>MRGSHHHHHTTGEDDESECVINYVEKAVNKLTLQMPYQLFIGGEFVDAEGSKTYNTINPTDGSVICQVSLAQVSDVDKAVAAAKEAFENGLWGKINARDRGRLL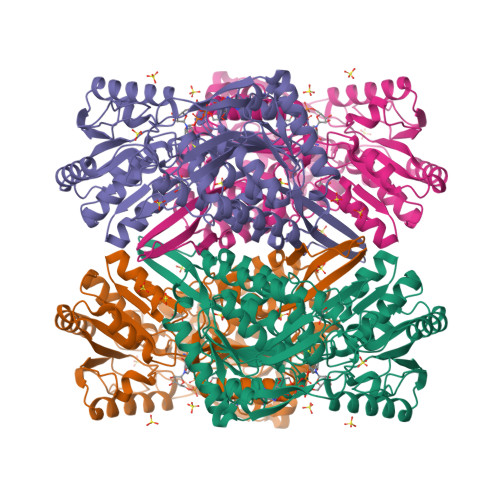YRLADVMEQHQEELATIEALDAGAVYTLALKTHVGMSIQTFRYFAGWCDKIQGATIPINQARPNRNLTLTKKEPVGVCGIVIPWNYPLMMLSWKTAACLAAGNTVVIKPAQVTPLTALKFAELTLKAGIPKGVVNILPGSGSLVGQRLSDHPDVRKIGFTGSTEVGKHIMKSCALSNVKKVSLELGGKSPLIIFADCDLNKAVQMGMSSVFFNKGENCIAAGRLFVEESIHNQFVQKVVEEVEKMKIGNPLERDTNHGPQNHEAHLRKLVEYCQRGVKEGATLVCGGNQVPRPGFFFQPTVFTDVEDHMYIAKEESFGPIMIISRFADGDVDAVLSRANATEFGLASGVFTRDINKALYVSDKLQAGTVFINTYNKTDVAAPFGGFKQSGFGKDLGEAALNEYLRIKTVTFEY[4x]>[2x]MAHTTTSMEIFGSTEQVWQLIGGFNSLPDWLPYIPSSKLTEGGRVRHLANPDGETIIE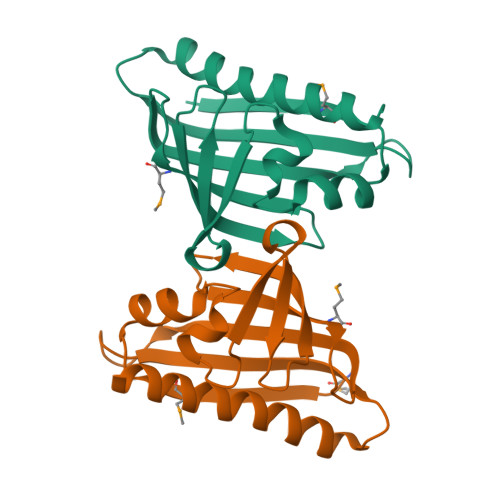RLEVFNDKERYYTYSIMNAPFPVTNYLSTIQVKEGTESNTSLVEWSGTFTPVAVSDEEAINLVHGIYSDGLKALQHAFLDLEHHHHHH4,4'-DIPYRIDYL DISULFIDE | C10 H8 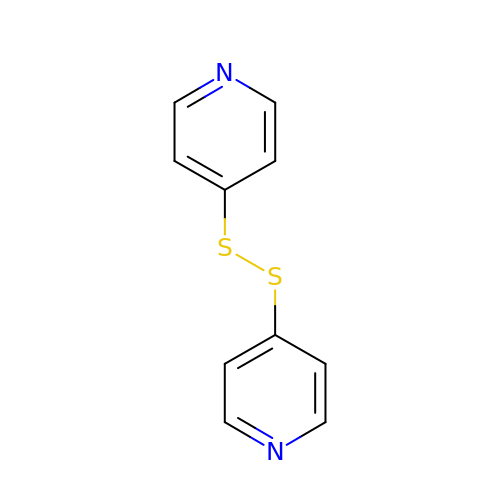N2 S2 | UHBAPGWWRFVTFS-UHFFFAOYSA-N(+)-2-[4-[(-1-ACETIMIDOYL-4-PIPERIDINYL)OXY]-3-(7-AMIDINO-2-NAPHTHYL)PROPIONIC ACID | C27 H30 N4 O3 | 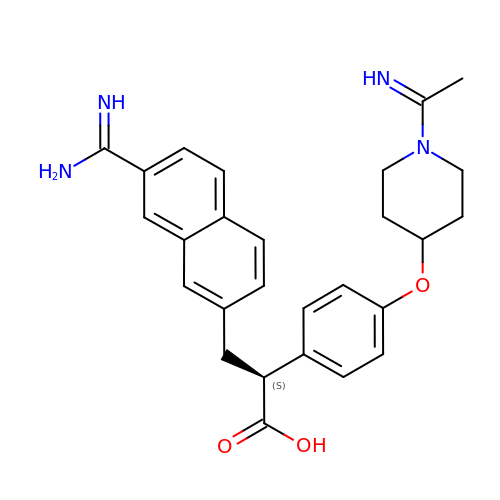FZLDAJVXFYWRCX-ISAGNRBTSA-N>[6x]S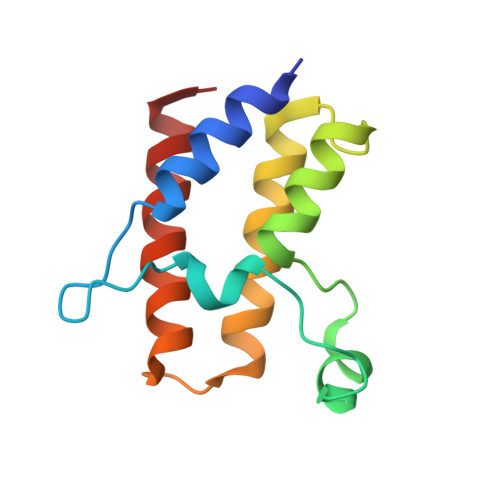MGIFPTVEKLVEEMREQLDEVDSHPRTSIFEKLPSKRDYPDYFKVIEKPMAIDIILKNCKNGTYKTLEEVRQALQTMFENARFYNEEGSWVYVDADKLNEFTDEWFKEHSS>CHCVILNDGNFIPVLGFGTALPLECPASKAKELTKIAIDAGFHHFDSASVYNTEDHVGEAIRSKIADGTVRREDIFYTSKVWCTSLHPELVRASLERSLQKLQFDYVDLYLIHYPMALKPGEENFPVDEHGKLIFDRVDLCATWEAMEKCKDAGLTKSIGVSNFNYRQLEMILNKPGLKYKPVCNQVECHPYLNQMKLLDFCKSKDIVLVAYGVLGTQRYGGWVDQNSPVLLDEPVLGSMAKKYNRTPALIALRYQLQRGIVVLNTSLKEERIKENMQVFEFQLSSEDMKVLDGLNRNMRYIPAAIFKGHPN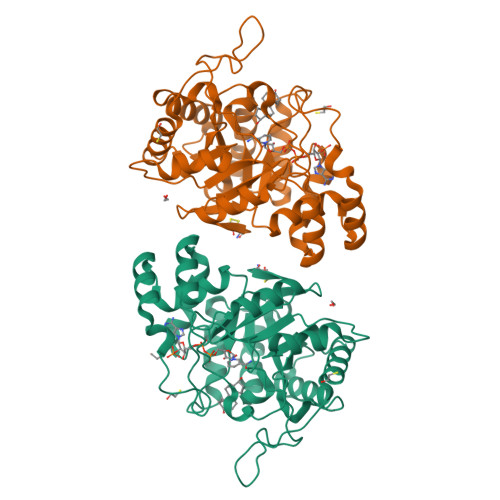WPFLDEY[2x]> MSGSHHHHHHSGSMSPSPIEEQATRLLKEVPLIDGHNDFPYMIRGWFRNDINGQDAHLYDMPIGQTDLQRLQKGLLGGQFWSAFVPCPKNPDKEVGSLEALRQTLQQLDVIHRLIERHPTILQFADSAASIWSSFRAGRVASLIGIEGLHQIADSVSALRMLHRLGVRYVTLTHNCHNAFADAATVSPELHGGLSRKGERLIRELNRMGMMIDLSHTSHEAQTQALRLSRAPVIYSHSSIYSLRAHARNVTDENLHLLHRNRGVVMICFLRELLASEADQATLAHV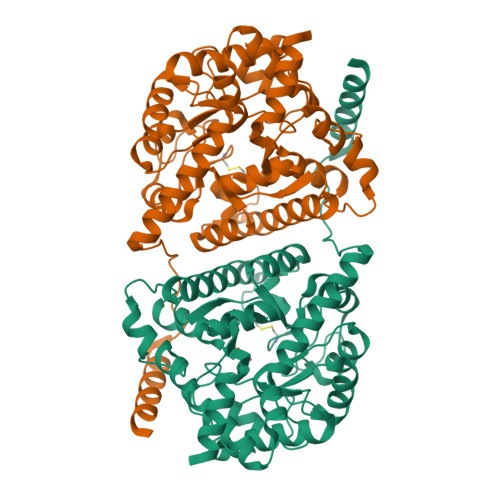IDHIIYAGTRIGYEHVGIGSDFDGMLRGPDGLHDVSCYPALVAGLLERGVSEEDVKRVMGLNVIRVLEEVERVAAELQGAGEECLCDELDEVWNEDIKEQLTRERERVRKLGPQ>[2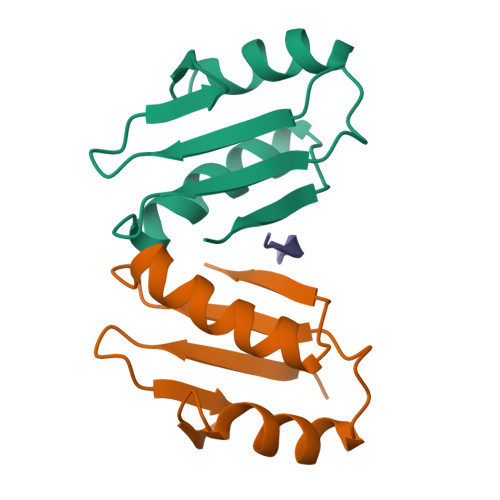x]RPEKPVYLSVKADNSMFIGNDPVTDETMITALNALTEGKKDTTIFFRADKTVDYETLMKVMDTLHQAGYLKIGLVGEETAKAK;> QPISVTMVTP> APEPWFFKNLSRKDAERQLLAPGNTHGSFLIRESESTAGSFCLSVRDFDQNQGEVVKHYKIRNL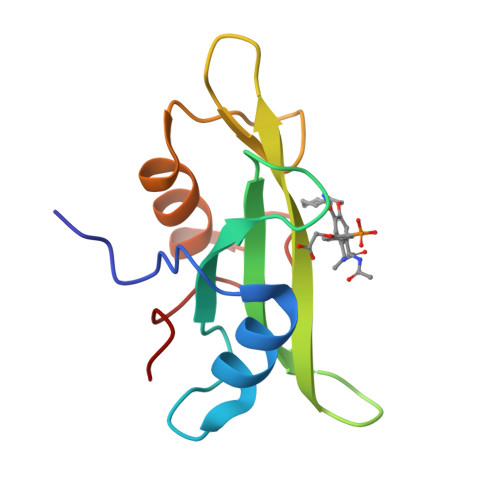DNGGFYISPRITFPGLHELVRHYTNASDGLCTRLSRPCQT(2R)-2-chloro-2-(difluoromethoxy)-1,1,1-trifluoroethane | C3 H2 Cl F5 O | 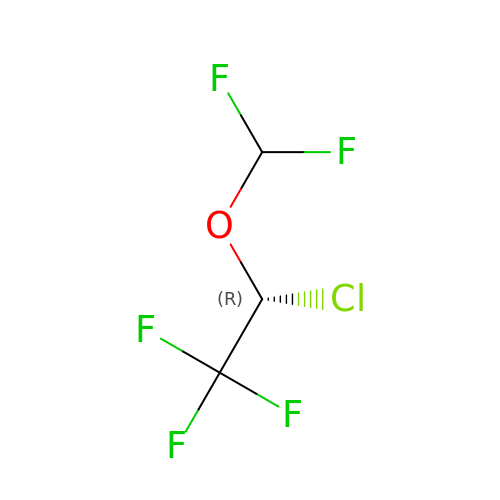PIWKPBJCKXDKJR-SFOWXEAESA-N>[2x]CG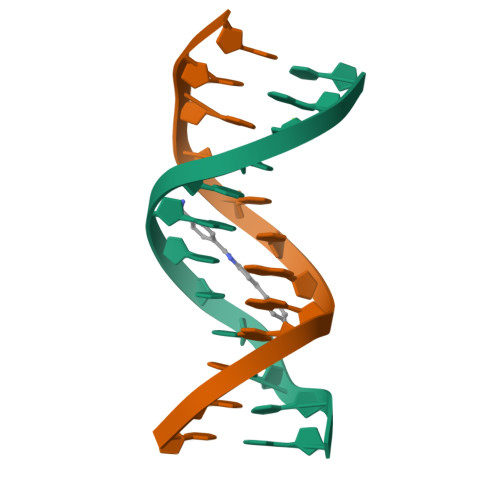CGAATTCGCG>MILSGKTISEKLTEKELEITPLTEEQIQPASVDLRLGPHFVTIDDSKEAVISFERPIRYREWTTSDETIVLPPHTFLLATTMETVKLPNHLTAFVEGRSSVGRLGLFIQNAGWVDPGFNGQITLELFNANRLPIELPIGRRICQLVFAEVTGEVAPYQG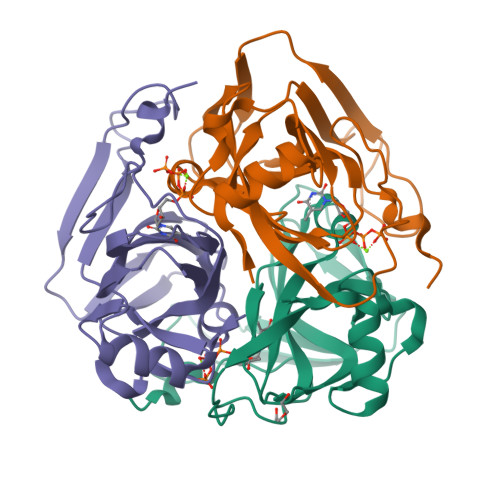KYLFQKGATMSEIYKDAF[6x]>[2x]HHH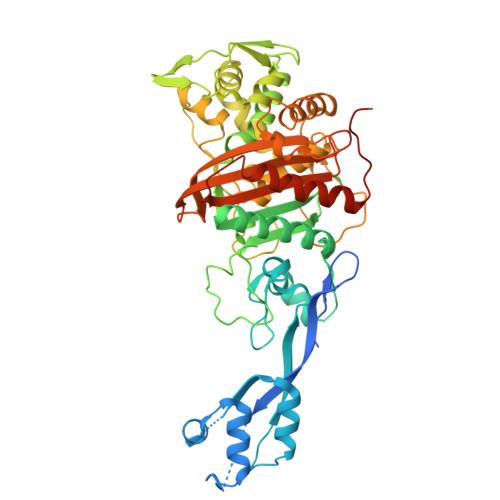HHHSSGENLYFQGHMDMRSLRVQEVPTARGMISDRSGRPLAVSVPVNAVWADPKELIEQGGISLDTRWKALSDALEIPLDQLATRINANPKGRFVYLARQVNPAIGDYIRKLKLPGIHLRQESRRYYPAGQVMAHIIGVTNIDGQGIEGVEKSFDRWLTGQPGERTVRKDHYGRVIEDISSVDSQAAHNLVLSVDERLQALVYRELNNAVAFNKAESGTAVLVDVNTGEVLAMANSPSYNPNNLTGTPKDAMRNRAITDIFEPGSTVKPMVVMTALQHGVVKENSVLNTLPYFVNGHQIKDVARYAELSVTGILQKSSNVGVSKLALAMPSSALVDTYSRFGFGKATNLGLVGESSGLYPKKQRWSDIERATFSFGYGLMVTPLQLARVYATIGSMGVYRPLSITRVDPPVAGERIFPEPLVRTVVHMMESVALPGGGGTKAAIKGYRIAIKTGTAKKVGPDGKYMDRYLAYTAGVAPASNPRFALVVVINDPQAGKYYGGAVSAPVFGAIMGGVLRTMNIEPDALPTGDKSELVINTKEGSGGRS> MNIKKFAKQATVLTFTTALLAGGATQAFAKETNQKPYKETYGISHITRHDMLQIPEQQKNEKYQVPEFDSSTIKNISSAKGLDVWASWPLQNADGTVANYHGYHIVFALAGDPKNADDTSIYMFYQKVGETSIDSWKNAGRVFKDSDKFDANDSILKDQTQEWSGSATFTSDGKIRLFYTDFSGKHYGKQTLTTAQVNVSASDSSLNINGVEDYKSIFDGDGKTYQNVQQFIDEGNYSSGDNHTLRDPHYVEDKGHKYLVFEANTGTEDGYQGEESLFNKAYYGKSTSFFRQESQKLLQSDKKRTAELANGALGMIEL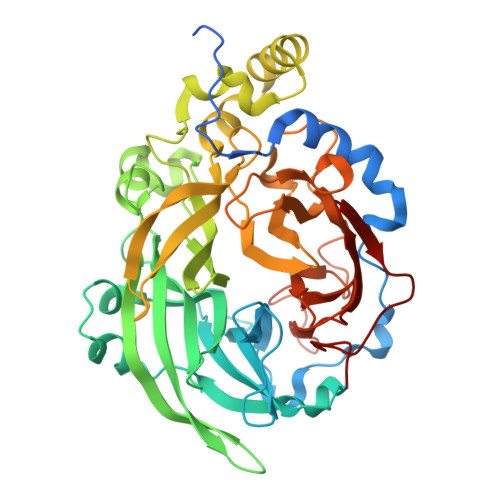NDDYTLKKVMKPLIASNTVTDEIERANVFKMNGKWYLFTDSRGSKMTIDGITSNDIYMLGYVSNSLTGPYKPLNKTGLVLKMDLDPNDVTFTYSHFAVPQAKGNNVVITSYMTNRGFYADKQSTFAPSFLLNIKGKKTSVVKDSILEQGQLTVNK>[2x]LAMTMEHKDRPLVRVILTNTGSHPV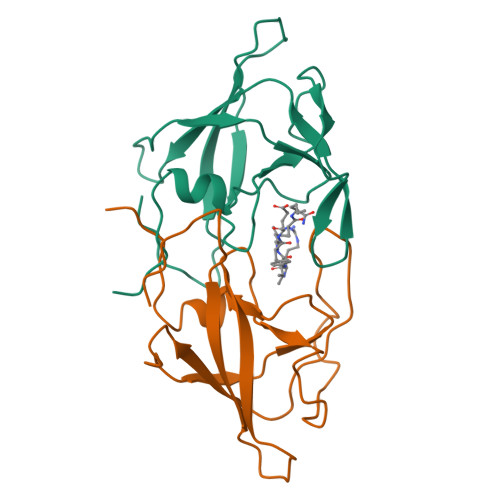KQRSVYITALLDTGADDTVISEEDWPTDWPVMEAANPQIHGIGGGIPVRKSRDMIELGVINRDGSLERPLLLFPLVAMTPVNILGRDCLQGLGLRLTNL> MASNEGVENRPFPYLTVDADLLSNLRQSAAEGLFHSFDLLVGKDAREAGIKFEVLLGVYTNAIQYVRFLETALAVSCVNTEFKDLSRMTDGKIQFRISVPTIAHGDGRRPSKQRTFIVVKNCHKHHISTEMELSMLDLEILHSIPETPVEYAEYVGAVKTVASALQFGVDALERGLINTVLSVKLRHAPPMFILQTLADPTFTERGFSKTVKSDLIAMFKRHLLEHSFFLDRAENMGSGFSQYVRSRLSEMVAAVSGESVLKGVSTYTTAKGGEPVGGVFIVTDNVLRQLLTFLGEEADNQIMGPSSYASFVVRGENLVTAVSYGRVMRTFEHFMARIVDSPEKAGSTKSDLPAVAAGVEDQPRVPISAAVIKLGNHAVAVESLQKMYNDTQSPYPLNRRMQYSYYFPVGLFMPNPKYTTSAAIKMLDNPTQQLPVEAWIVNKNNLLLAFNLQNALKVLCHPRLHTPAHTLNSLNAAPAPRDRRETYSLQHRRPNHMNVLVIVDEFYDNKYAAPVTDIALKCGLPTEDFLHPSNYDLLRLELHPLYDIYIGRDAGERARHRAVHRLMVGNLPTPLAPAAFQEARGQQFETATSLAHVVDQAVIETVQDTAYDTAYPAFFYVVEAMIHGFEEKFVMNVPLVSLCINTYWERSGRLAFVNSFSMIKFICRHLGNNAISKEAYSMYRKIYGELIALEQALMRLAGSDVVGDESVGQYVCALLDPNLLPPVAYTDIFTHLLTVSDRAPQIIIGNEVYADTLAAPQFIERVGNMDEMAAQFVALYGYRVNGDHDHDFRLHLGPYVDEGHADVLEKIFYYVFLPTCTNAHMCGLGVDFQHVAQTLAYNGPAFSHHFTRDEDILDNLENGTLRDLLEISDLRPTVGMIRDLSASFMTCPTFTRAVRVSVDNDVTQQLAPNPADKRTEQTVLVNGLVAFAFSERTRAVTQCLFHAIPFHMFYGDPRVAATMHQDVATFVMRNPQQRAVEAFNRPEQLFAEYREWHRSPMGKYAAECLPSLVSISGMTAMHIKMSPMAYIAQAKL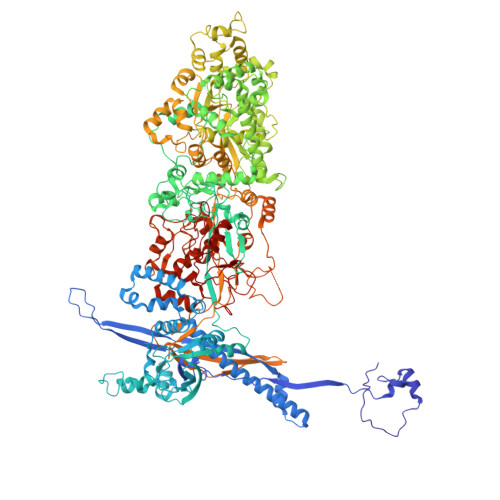KIHPGVAMTVVRTDEILSENILFSSRASTSMFIGTPNVSRREARVDAVTFEVHHEMASIDTGLSYSSTMTPARVAAITTDMGIHTQDFFSVFPAEAFGNQQVNDYIKAKVGAQRNGTLLRDPRTYLAGMTNVNGAPGLCHGQQATCEIIVTPVTADVAYFQKSNSPRGRAACVVSCENYNQEVAEGLIYDHSRPDAAYEYRSTVNPWASQLGSLGDIMYNSSYRQTAVPGLYSPCRAFFNKEELLRNNRGLYNMVNEYSQRLGGHPATSNTEVQFVVIAGTDVFLEQPCSFLQEAFPALSASSRALIDEFMSVKQTHAPIHYGHYIIEEVAPVRRILKFGNKVVF> MVDINLFREE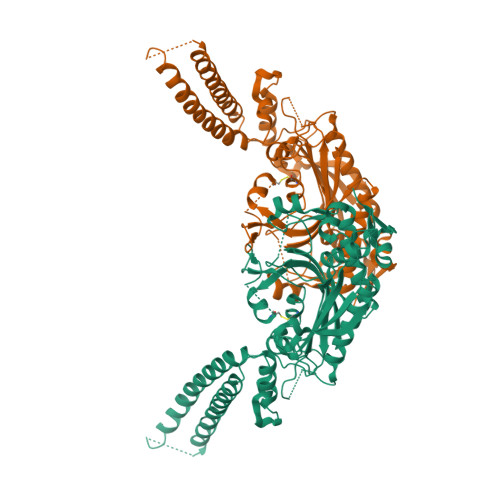KGNNPEIIRESQRRRFASVEIVDEIIKLDKEWRQRQFEVDSFRKEFNKLNKQVAQLKIKKEDASEIIQQTEKNKQDSTAKEAEVREAYAALKAKLEQVGNLVHDSVPVDKDEANNLVIKLWGEKRFSTPGLKLKNHVDLVELLGIADTKRGAEIAGARGFFLKGDGLMLNQALINFGLTFLKKRGFTGLQPPFFMRKDVMAKCAQLAQFDEELYKVTGEGDDKYLIATAEQPLCAYHIDEWIHPTELPLRYAGYSSCFRKEAGSHGRDTLGIFRVHQFEKIEQFCITGPNENASWEMLDEMMKNSEDFYQALKLPYQIVSIVSGALNDAAAKKYDLEAWFPSSETFRELVSCSNCTDYQARRLEIRYGQKKSNEQTKQYVHMLNSTLTATERTICCILENYQREDGVDIPEVLQPFMGGETFLPFKAKPVVADTKGKKSKAAAALE> MKFPQLCKFCDVRFSTCD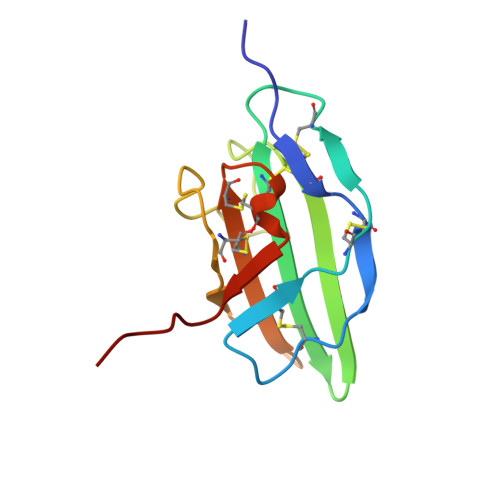NQKSCMSNCSITSICEKPQEVCVAVWRKNDENITLETVCHDPKLPYHDFILEDAASPKCIMKEKKKPGETFFMCSCSSDECNDNIIFSEEYNT> GSMAVTRYVDNNFCGPD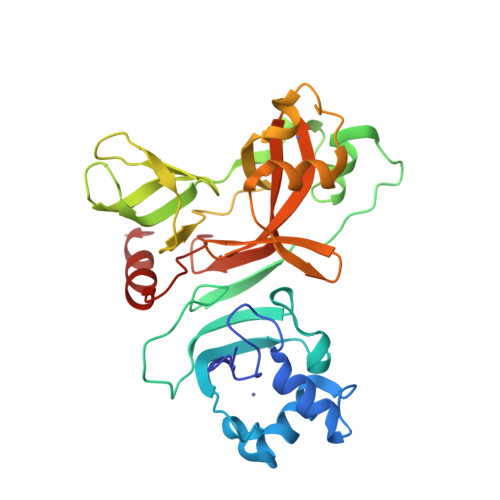GYPLDCIKDFLARAGKSMCTLSEQLDYIESKRGVYCCRDHDHEIAWFTERSDKSYEHQTPFEIKSAKKFDTFKGECPKFVFPLNSKVKVIQPRVEKKKTEGFMGRIRSVYPVASPQECNNMHLSTLMKCNHCDEVSWQTCDFLKATCEHCGTENLVIEGPTTCGYLPTNAVVKMPCPACQDPEIGPEHSVADYHNHSNIETRLRKGGRTRCFGGCVFAYVGCYNKRAYWVPRASADIGSGHTGITGDNVETLNEDLLEILSR> MKVQAENAARLGRQVLGLLPPPTHRVSLTRGPEFARGVRDLLSKYAASTRPTVGSLHEALRQAPFRQPTYGDFLVYSQTFSPQEPLGTFLFSFKQEDNGSSMDMLLTPTSLFMLSGMEAAKAPQTHKVAGVWYGSGSGLADFIPNLSELMDTGEFHTLLTPVGPMVQSVHSTFVTKVTSAMKGVGLARDEPRAHVGLTLPCDMLVDLDESCPMVQRREP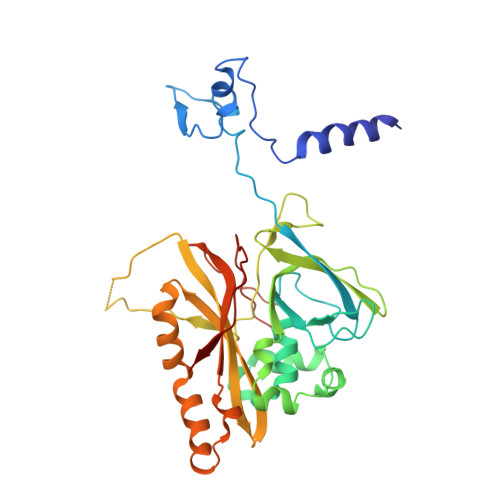AGLNVTIYASLVYLRVNQRPSMALTFFQSGKGFAEVVAMIKDHFTDVIRTKYIQLRHELYINRLVFGAVCTLGTVPFDSHPVHQSLNVKGTSLPVLVFANFEAACGPWTVFL(2R,3S)-3-methyl-4-methylidene-2-[(2S,3R)-3-oxidanyl-1-oxidanylidene-butan-2-yl]-2,3-dihydropyrrole-5-carboxylic 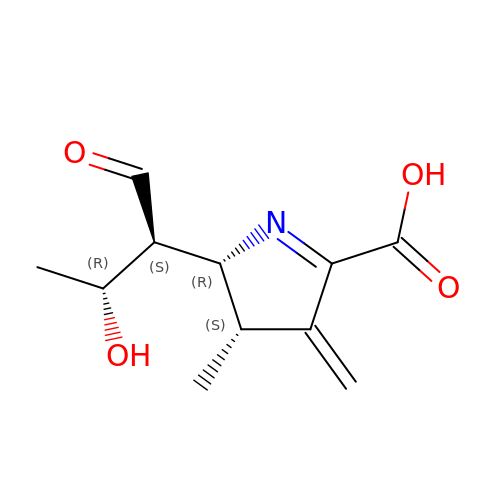acid | C11 H15 N O4 | GGYAWCWTCNLFOB-KDBVAPGDSA-N>GGHMAIKFNIKESKILNGVYIITPNKFSDLRGDIWTAFTDEYLSNLVPNGIKFKHDKFINSHFNVLRGIHGDVKTYKLVTCVYGEVHQVVVDCRKDSPTYLKWEKFIISPRNQQLILLPPNMGNSHYVSSKEAVYYYKLAYKGEYLDAPDQFTYAWNDKRIAIDWPTNSPILSER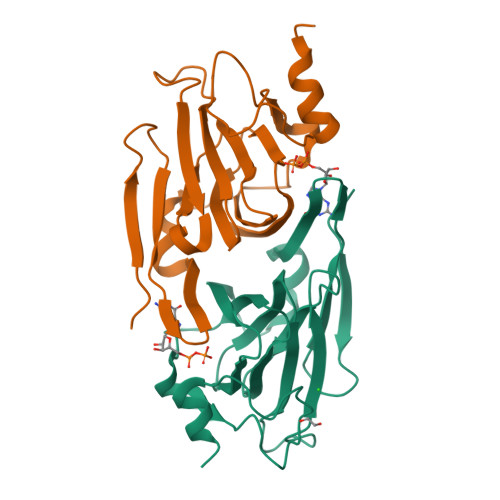DILAMNKDK[2x]> MVRVPRERSGTRSALGEASTYPVGAMTSQHDDQMTFYEAVGGEETFTRLARRFFEGVAADPVLRPMFPEEDLGPAEERLRLFLMQYWGGPETYSERRGHPRLRMRHEPYRIGAEERDRFLTHMRAAVDDLALPAHLEQQLWEYLVYA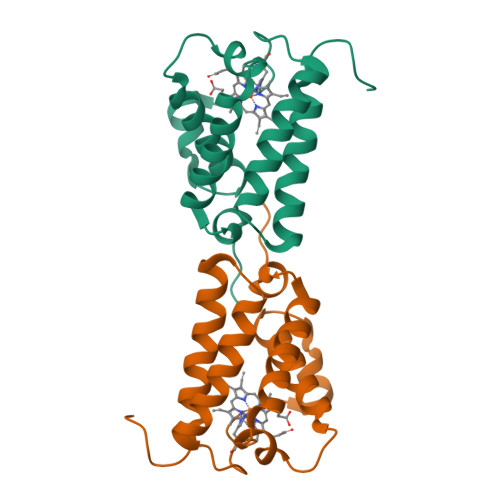AYAMVNVPEDAQPPMVQ>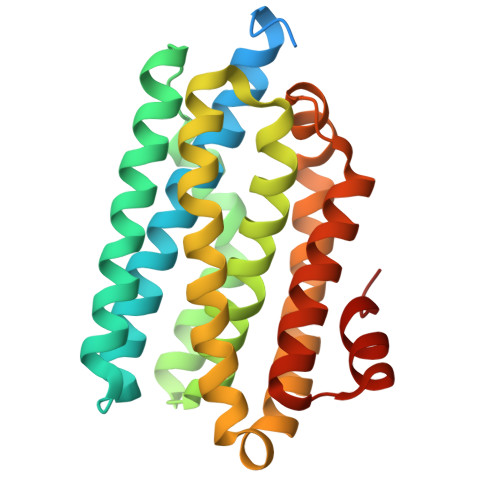 MRTPWDPPNPTFSLSSVSGDRRLMPQLEASLELDFQSESYKDAYSRINAIVIEGEQEAFDNYNRLAEMLPDQRDELHKLAKMEQRHMKGFMACGKNLSVTPDMGFAQKFFERLHENFKAAAAEGKVVTCLLIQSLIIECFAIAAYNIYIPVADAFARKITEGVVRDEYLHRNFGEEWLKANFDASKAELEEANRQNLPLVWLMLNEVADDARELGMERESLVEDFMIAYGEALENIGFTTREIMRMSAYGLAAV> VVEAVENAVARVADT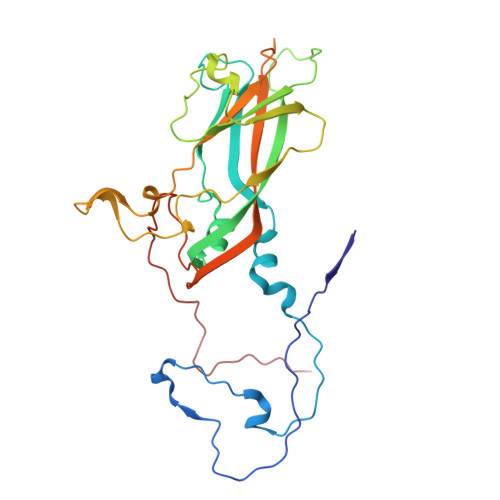ISSGPSNSQAVPALTAVETGHTSQVTPSDTIQTRHVRNYHSRSESSIENFLCRSACVYMGEYHTTNTDTSKLFASWTINARRMVQMRRKLELFTYVRFDMEVTFVITSKQDQGTQLGQDMPPLTHQIMYIPPGGPIPKSVTDYTWQTSTNPSIFWTEGNAPPRMSIPFISIGNAYSNFYDGWSHFSQNGVYGYNTLNHMGQIYVRHVNGSSPLPMTSTVRMYFKPKHVKVWVPRPPRLCQYKNASTVNFTPTNITEKRQSINYIPETVKP(2~{S})-2-[[(2~{S})-4-methyl-2-[[oxidanyl-[(1~{S})-2-phenyl-1-(phenylmethoxycarbonylamino)ethyl]phosphoryl]amino]pentanoyl]amino]propanoic 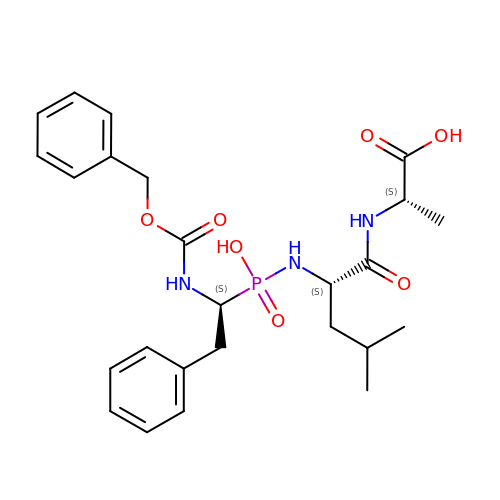acid | C25 H34 N3 O7 P | PREBTZMCCRSQJI-NYVOZVTQSA-N> GAMTKPRFTTGLVY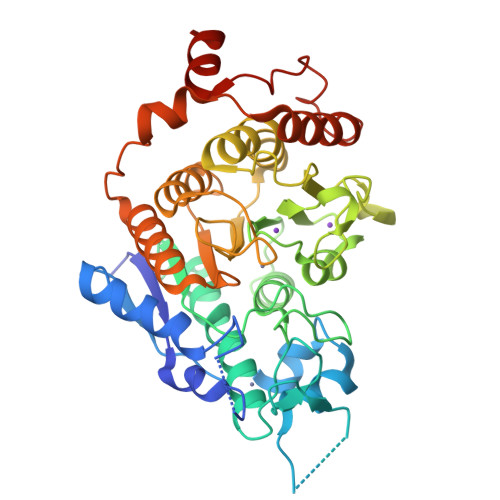DTLMLKHQCTCGSSSSHPEHAGRIQSIWSRLQETGLRGKCECIRGRKATLEELQTVHSEAHTLLYGTNPLNRQKLDSKKLLGSLASVFVRLPCGGVGVDSDTIWNEVHSAGAARLAVGCVVELVFKVATGELKNGFAVVRPPGHHAEESTPMGFCYFNSVAVAAKLLQQRLSVSKILIVDWDVHHGNGTQQAFYSDPSVLYMSLHRYDDGNFFPGSGAPDEVGTGPGVGFNVNMAFTGGLDPPMGDAEYLAAFRTVVMPIASEFAPDVVLVSSGFDAVEGHPTPLGGYNLSARCFGYLTKQLMGLAGGRIVLALEGGYDLTAICDASEACVSALLGNELDPLPEKVLQQRPNANAVRSMEKVMEIHSKYWRCLQRTTSTAGRSLIEAQTCENEEAETVT> GVGRLDDLKRSPLFQNVPEDAMREALKVVTERNFQPDELVVEQDAEGEALHLVTTGVVRVSRVSLGGRERVLGDIYAPGVVGETAVLAHQERSASVRALTPVRTLMLHREHFELILRRHPRVLWNLAEMLARRVTFLNDELIAFGQNTEAALTHVFANLYRQRLAA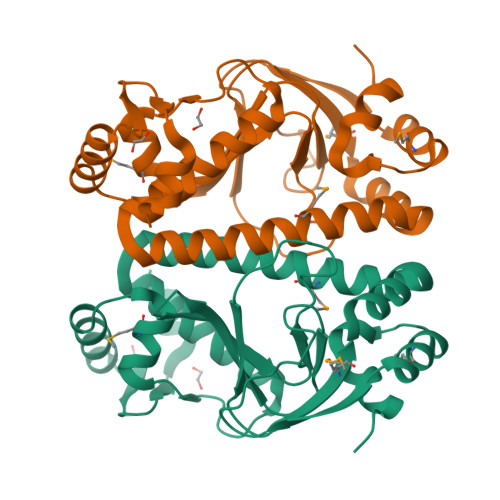GVPQPEVLPLGTQDIMARTSSSRETVSRVLKRLEAHNILEVSPRSVTLLDLAALEALSFEGAETD> MGPAFEFAVAMMKRNSSTVKTEYGEFTMLGIYDRWAVLPRHAKPGPTILMNDQEVGVLDAKELVDKDGANLELTLLKLNRNEKFRDIRGFLAKEEVEVNEAVLAINTSKFPNMYIPVGQVTEYGFLNLGGTPTKRMLMYNFPTRAGQCGGVLMSTGKVLGIHVGGNGHQGFSAALLKHY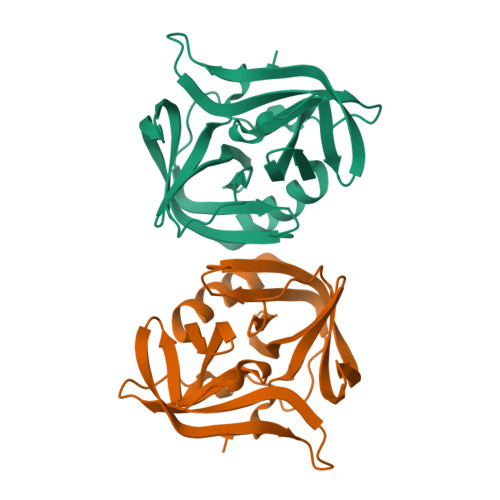FNDEQ>[2x]MSTDKITFLLNWQPTPYHIPIFLAQTKGYFKEQGLDMAILEPTNPSDVTELIGSGKVDMGLKAMIHTLAAKARGFPVTSVASLLDEPFTGVLYLKGSGITEDFQSLKGKKIGYVGEFGKIQIDELTKHYGMKPEDYTAVRCGMNVAKYIIEGKIDAGIGIECMQQVELEEYLAKQGRPASDAKMLRIDKLACLGCCCFCTVLYICNDEFLKKNPEKVRKFLKAIKKAT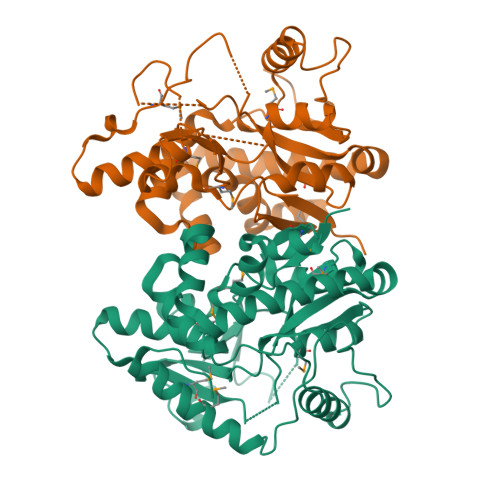DYVLADPVKAWSGYIDFKPQLNNDLSYKQYQRCYAYFSSSLYNVHRDWKKVTGYGKRLAILPPDYVSNYTNEYLSWPEPEEVSDPLEATRLMAIHQEKCRQEGTFKRLALPAHHHHHH>[2x]GTEDLYFQSHMTIAVT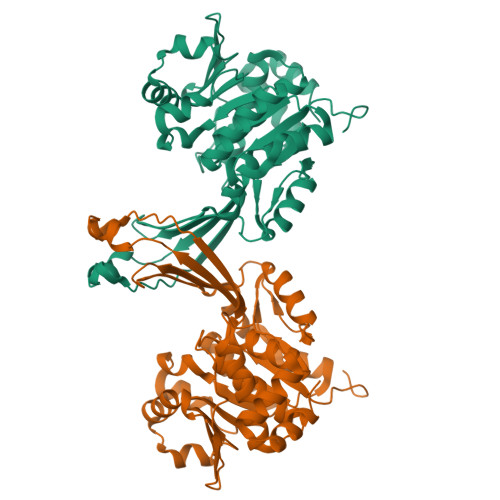GSIATDHLMRFPGRFSEQLLPEHLHKVSLSFLVDDLVMHRGGVAGNMAFAIGVLGGEVALVGAAGADFADYRDWLKARGVNCDHVLISETAHTARFTCTTDVDMAQIASFYPGAMSEARNIKLADVVSAIGKPELVIIGANDPEAMFLHTEECRKLGLAFAADPSQQLARLSGEEIRRLVNGAAYLFTNDYEWDLLLSKTGWSEADVMAQIDLRVTTLGPKGVDLVEPDGTTIHVGVVPETSQTDPTGVGDAFRAGFLTGRSAGLGLERSAQLGSLVAVLVLESTGTQEWQWDYEAAASRLAGAYGEHAAAEIVAVLA> MHHHHHHSRY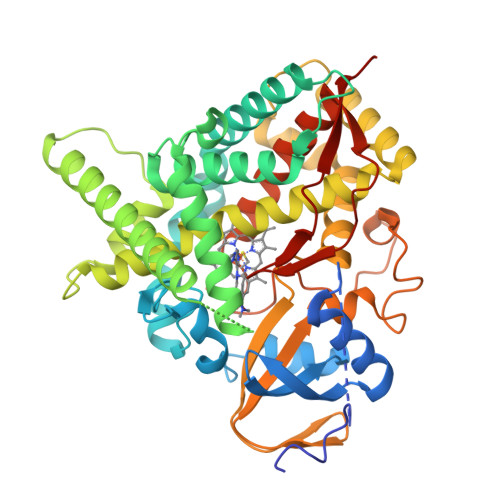EHIPGPPRPSFLLGHLPCFWKKDEVGGRVLQDVFLDWAKKYGPVVRVNVFHKTSVIVTSPESVKKFLMSTKYNKDSKMYRALQTVFGERLFGQGLVSECNYERWHKQRRVIDLAFSRSSLVSLMETFNEKAEQLVEILEAKADGQTPVSMQDMLTYTAMDILAKAAFGMETSMLLGAQKPLSQAVKLMLEGITASRNTLAKFLPGKRKQLREVRESIRFLRQVGRDWVQRRREALKRGEEVPADILTQILKAEEGAQDDEGLLDNFVTFFIAGHETSANHLAFTVMELSRQPEIVARLQAEVDEVIGSKRYLDFEDLGRLQYLSQVLKESLRLYPPAWGTFRLLEEETLIDGVRVPGNTPLLFSTYVMGRMDTYFEDPLTFNPDRFGPGAPKPRFTYFPFSLGHRSCIGQQFAQMEVKVVMAKLLQRLEFRLVPGQRFGLQEQATLKPLDPVLCTLRPRGWQPA> QQLLKGLSLS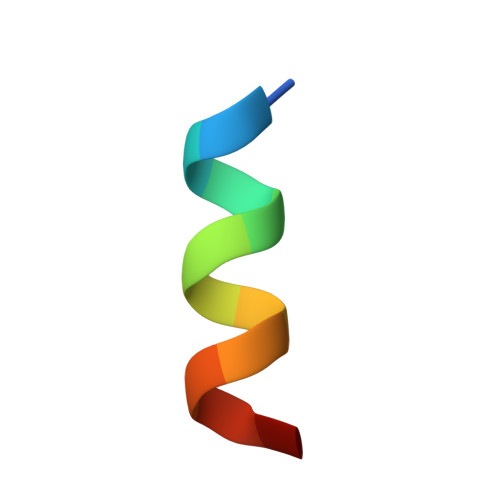FSK> XVNAKQXHR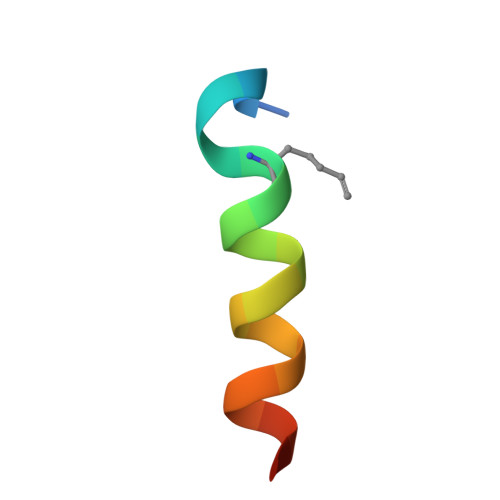IXKRRQARAKLX> MNGIYIWKIGNFGMHLKCQEEEKPVVIHSPGFYTGKPGYKLCMRLHLQLPTAQRCANYISLFVHTMQGEYDSHLPWPFQGTIRLTILDQSEAPVRQNH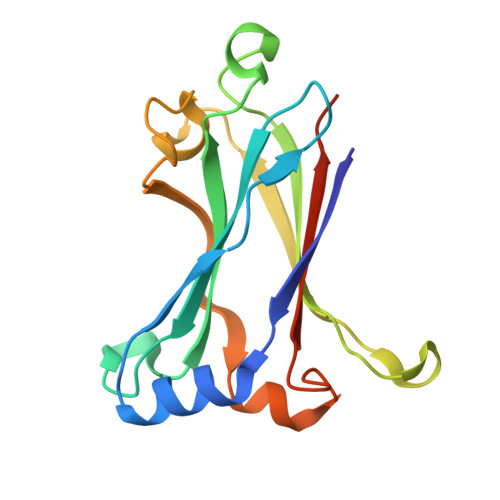EEIMDAKPELLAFQRPTIPRNPKGFGYVTFMHLEALRQRTFIKDDTLLVRCEVSTLEHHHHHH>MLIQAVGVNLPPSYVCLEGPLGGERPRAQGDEMLMQRLLPAVREALDEAAVKPEEIDLIVGLALSPDHLIENRDIMAPKIGHPLQKVLGANRAHVFDLTDSSLARALYVVDTLASDQGYRNVLVVRGESSQGLEVDSESGFALADGALALLCRPTGKAAFRRGALGGDPAQEWLPLSIPLNTDIRQVGDVKGHLNLPAQPGLPEAVRAGFTRLAGDFPQLNWVREEWFGQGRPDGRCLGPFELASQLRAAQRDRLDELLLISFDPFGMVVEGVTLELAGEAHA[4x];>[4x]SAGHKVKLAAITCELPARSYENDDPVFAAVPDLSESWWQFWGVNRRGYFDPRNGENEFSLVVRAAERLLRSSDTAPDSVDMLICSASSPIMTDAGDVLPDLRGRLYPRMANVLSKQLGLSRALPLDSQMEAASFLLNLRLAASMIRQGKAEKVLVVCSEYISNLLDFTSRTSTLFADGCAVALLTRGDDDSCDLLASAEHSDATFYEVATGRWRLPENPTGEAKPRLYFSLFSDGQNKMASFVPTNVPIAMRRALEKAGLGSDDIDYFVFHQPAPFLVKAWAEGIGARPEQYQLTMGDTGVMISVSIPYTLMTGLREGKIRPGDRIVMAGAATGWGFAAQ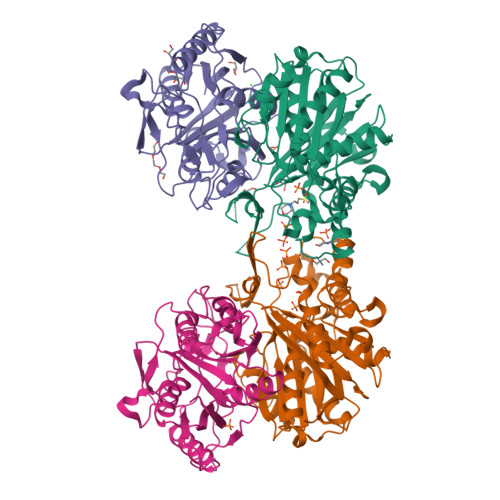VWQLGEVLVC> QTSVSPSKVILPRGGSVLVTCSTSCDQPKLLGIETPLPKKELLLPGNNRKVYELSNVQEDSQPMCYSNCPDGQSTAKTFLTVYWTPERVELAPLPSWQPVGKNLTLRCQVEGGAPRANLTVVL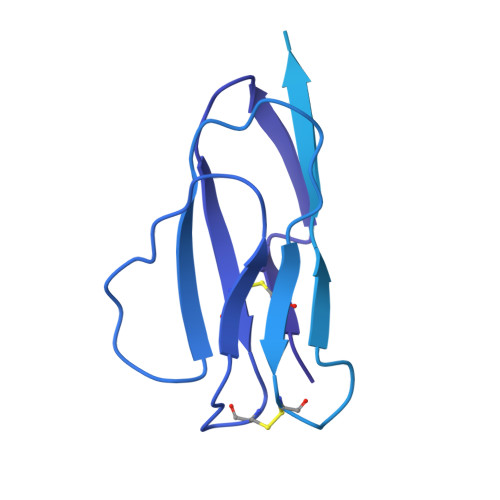LRGEKELKREPAVGEPAEVTTTVLVRRDHHGANFSCRTELDLRPQGLELFENTSAPYQLQTFVLPATPPQLVSPRVLEVDTQGTVVCSLDGLFPVSEAQVHLALGDQRLNPTVTYGNDSFSAKASVSVTAEDEGTQRLTCAVILGNQSQETLQTVTIYSFPAPNVILTKPEVSEGTEVTVKCEAHPRAKVTLNGVPAQPLGPRAQLLLKATPEDNGRSFSCSATLEVAGQLIHKNQTRELRVLYGPRLDERDCPGNWTWPENSQQTPMCQAWGNPLPELKCLKDGTFPLPIGESVTVTRDLEGTYLCRARSTQGEVTRKVTVNVLSPRYE> DKCKEREEKIILVSSANEIDVRPCPLNPNEHKGTITWYKDDSKTPVSTEQASRIHQHKEKLWFVPAKVEDSGHYYCVVRNSSYCLRIKISAKFVEN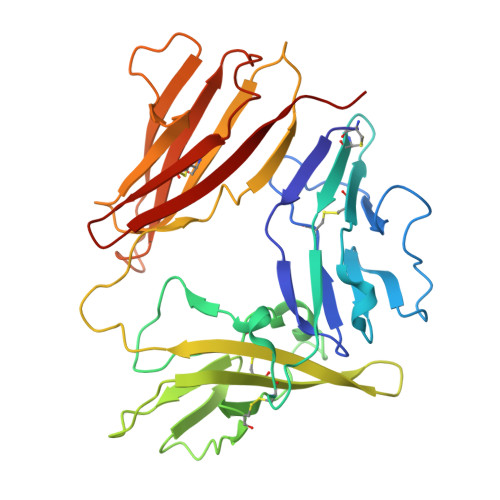EPNLCYNAQAIFKQKLPVAGDGGLVCPYMEFFKNENNELPKLQWYKDCKPLLLDNIHFSGVKDRLIVMNVAEKHRGNYTCHASYTYLGKQYPITRVIEFITLEENKPTRPVIVSPANETMEVDLGSQIQLICNVTGQLSDIAYWKWNGSVIDEDDPVLGEDYYSVENPANKRRSTLITVLNISEIESRFYKHPFTCFAKNTHGIDAAYIQLIYPVT> QCRLRPWLEEQIQSGRYPGVQWLDQSARVFQIPWKHAARHGWN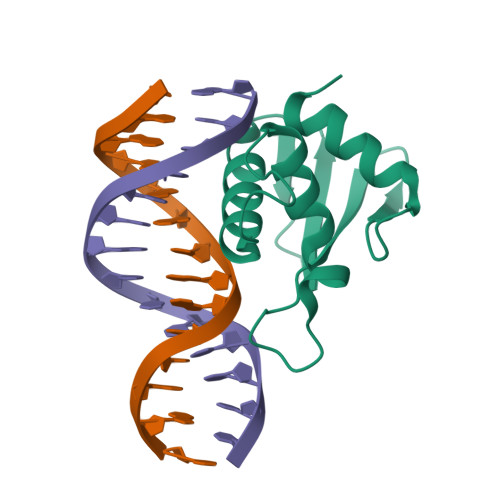IDKDATLFRNWAIHTGRYKPGIDKPDPKTWKANFRCALNSLTDVKELQDRSIKKGHNAFRVYALL>[2x]MNHKVHHHHHHMTTSKEDNDMINKLNKVFKNKLSNTGNIFVKYSNAYKVNAALMAAISIHETGNGSSSLCKN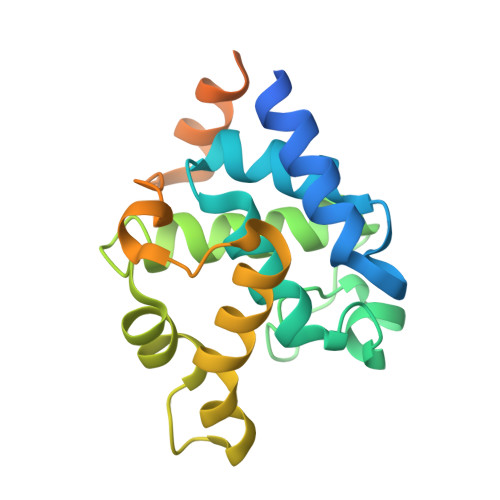KNNFFGMKGMSFGSVDEGIKRGISNLSRNYIHTGRKTLESIRDKYAPLYDSPLNKDWVPGVGKFYKQITGNAYSSNSAGTGVGSNEEAEKNLKDTTYQVQNNNSNTLTNNNSKVSKVIQEAKNQLGKPY6-benzyl-N4-((1r,3r)-3-hydroxycyclobutyl)-N2-methylpyridine-2,4-dicarboxamide | C19 H21 N3 O3 | 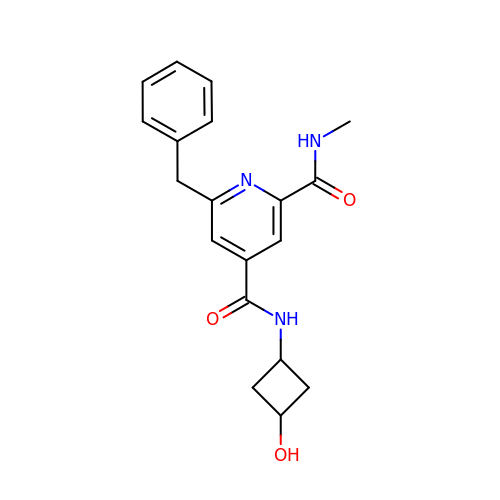FQRNJZDJWMGBEX-WKILWMFISA-N(1R,3S,4R,5S,6R)-2,4,5,6-tetrakis(phosphonooxy)cyclohexane-1,3-diyl bis[trihydrogen 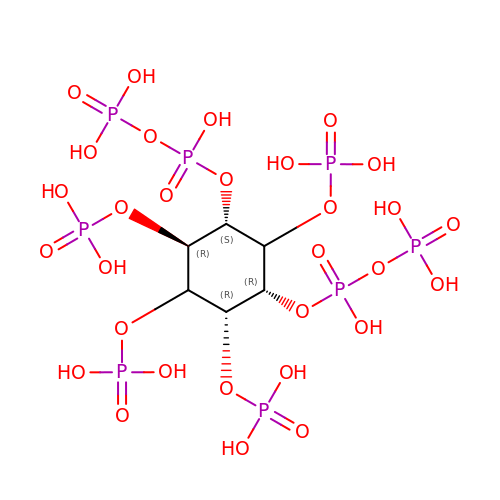(diphosphate)] | C6 H20 O30 P8 | HHQOOERQSFJGEP-SLWYWOEDSA-N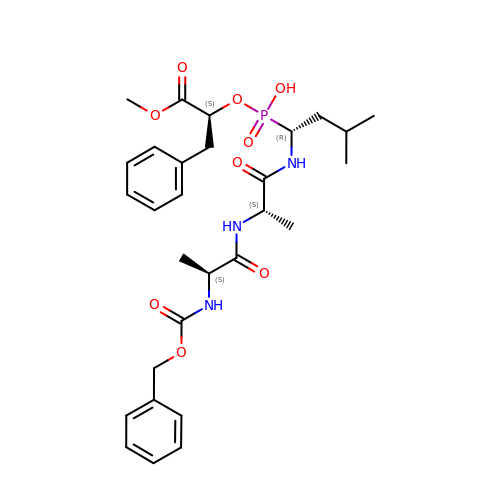N-[(benzyloxy)carbonyl]-L-alanyl-N-{(1S)-1-[(R)-[(1R)-1-benzyl-2-methoxy-2-oxoethoxy](hydroxy)phosphoryl]-3-methylbutyl}-L-alaninamide | C29 H40 N3 O9 P | VWCUANLUSQBJLX-WIHVIGOGSA-N> G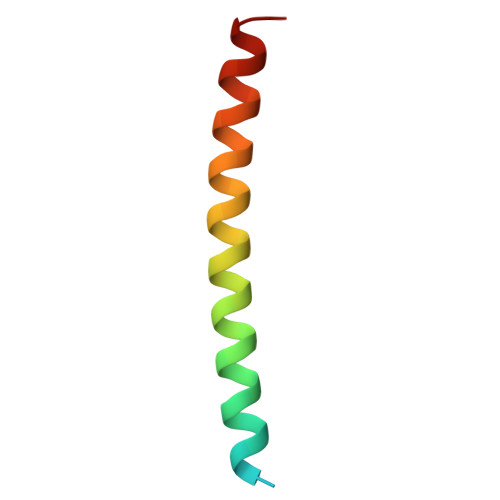SKDAELQEREYHLKELREQLAKQTVAIAELTEELQSKCIQLNKLQ>MGRYSGKTCRLLFMLVLTVAFFVAELVSGYLGNSIALLSDSFNMLSDLISLCVGLSAGYIARRPTRGFSATYGYARAEVVGALSNAVFLTALCFTIFVEAVLRLARPERIDDPELVLIVGVLGLLVNVVGLLIFQDCAAWFACCLRGRSRRLQQRQQLAEGCVPGAFGGPQGAEDPRRAADPTAPGSDSAVTLRGTSVERKREKGATVFANVAGDSFNTQNEPEDMMKKEKKSEALNIRGVLLHVMGDALGSVVVVITAIIFYVLPLKSEDPCNWQCYIDPSLTVLMVIIILSSAFPLIKETAAILLQMVPKGVNMEELMSKLSAVPGISSVHEVHIWELVSGKIIATLHIKYPKDRGYQDASTKIREIFHHAGIHNVTIQFENVDLKEPLEQKDLLLLCNSPCISKGCAKQLCCPPGA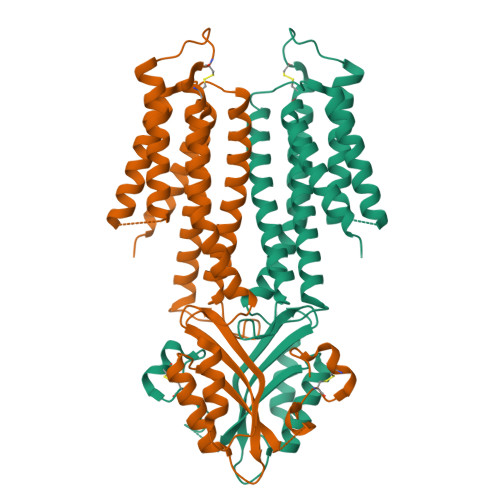LPLAHVNGCAEHNGGPSLDTYGSDGLSRRDAREVAIEVSLDSCLSDHGQSLNKTQEDQCYVNRTHF[2x]>[2x]RLKALQQKQTQTTSAAEDKTKPLEEAFDWD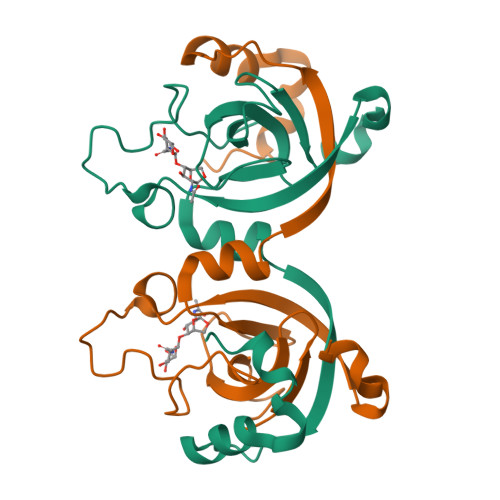EYPVQRVTATGYTAGAESTGKNPGDPLYGLTYSGVKVKRDLYSTVAADPSVFPIGTILFIPNYGLGVVADTGSAIKGNRLDLYFETVKDVYNEWGKKTLDVYVIKKGTGKITEDELEKLNETKSLQVFRNQYKTVK> MQPFDSGHDDLVHDVVYDFYGRHVATCSSDQHIKVFKLDKDTSNWELSDSWRAHDSSIVAIDWASPEYGRIIASASYDKTVKLWEEDPDQEECSGRRWNKLCTLNDSKGSLYSVKFAPAHLGLKLACLGNDGILRLYDALEPSDLRSWTLTSEMKVLSIPPANHLQSDFCLSW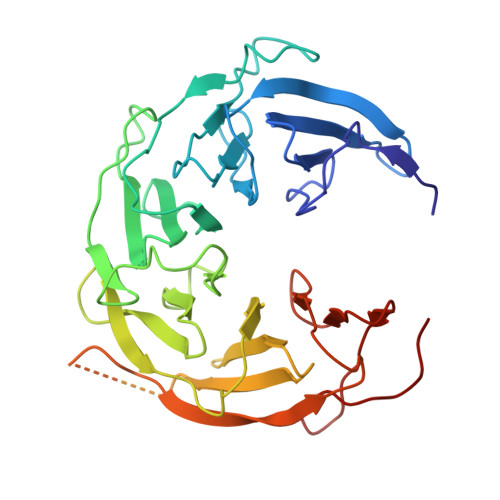CPSRFSPEKLAVSALEQAIIYQRGKDGKLHVAAKLPGHKSLIRSISWAPSIGRWYQLIATGCKDGRIRIFKITEKLSPLASEESLTNSNMFDNSADVDMDAQGRSDSNTEEKAELQSNLQVELLSEHDDHNGEVWSVSWNLTGTILSSAGDDGKVRLWKATYSNEFKCMSVITAQQ> AATSAAKKYDLFGYEVDTNT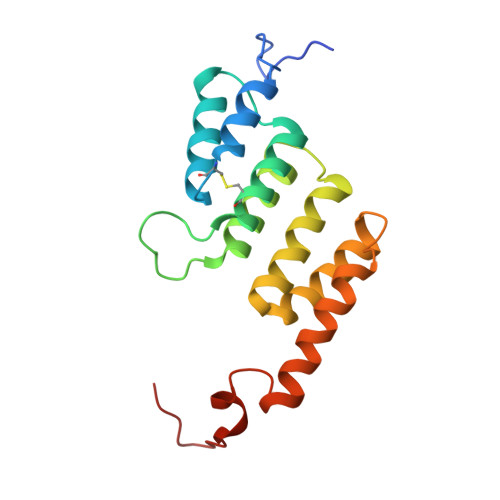APWIEKIKKCKYYDEAGEVLVNMNVSNCPPDIATYNATLQCIYQSPSKQSTPVDNESKFCAMMDLLEEMQHRNRLKPNEESWTWVMKECVKSGQFRLGYCIQQVMETECKGCPADLVKANEANAQKAKTEGKEHPGHLSQQAGLFDVKVE1-cyclobutyl-N-[3-(dimethylamino)propyl]-2-(3,4,5-trimethoxyphenyl)-1H-1,3-benzimidazole-6-carboxamide | C26 H34 N4 O4 | 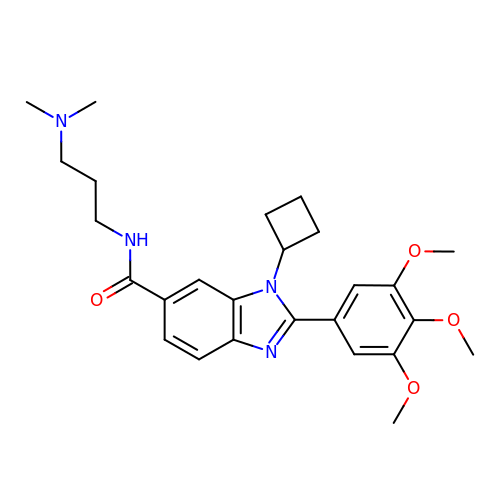QSAGTNCQQMIGRY-UHFFFAOYSA-N> 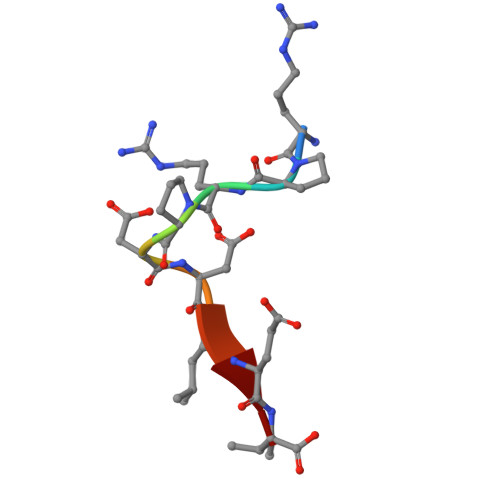RPRPDDLEI>GHMAASTAVAPVENGAAPAVAHKRTFAQRHSELIKHFPSTMGVDDFMGRVEVALAGFGFTGDNTIAMTNLCRDEVTQVLKDKIEAIFGSSFNTNGLGGVLTCGVTGMKAGLSHSPVCNGGRERYVFFAFPHIAINSEGEMGALSRPGRPKQSCACGALLAILNAFKVDGVEKSCKVPGVHDPLDPELTILQQRLARRVRYEKLDVSKLDLPGLTSVAERTITDDLEYLIEKAVDPAVADYAVITGVQIHNWGKELSASGDASIEFVAPAKCYTVVN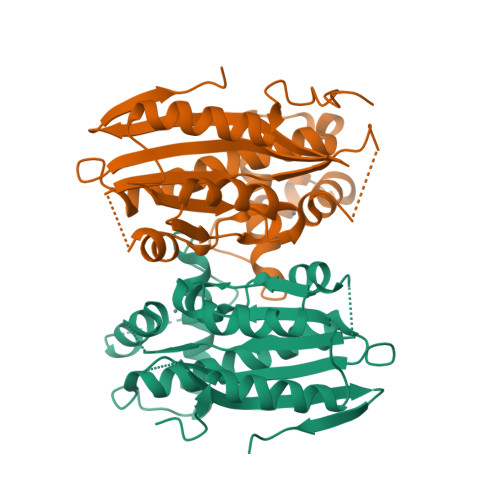GLKTYIDLPQVPALSPRQIQT[2x]>SNAEK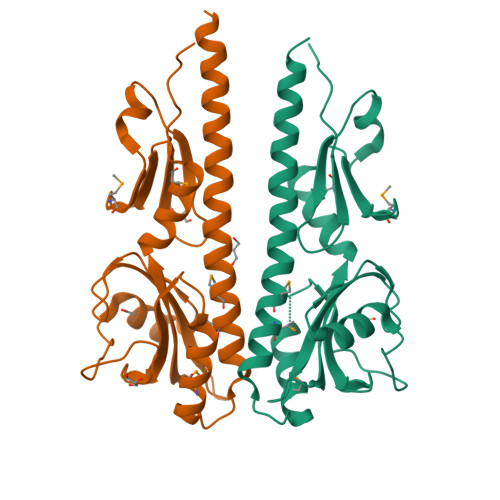EKDTIAAEHKQEASVLLNLHRNKINYLIGETMARMTSLSIAIDRPVDIKKMQSILEKTFDSEPRFSGLYFLNAKGDVTASTTELKTKVNLADASFFIKAKETKKTVISDSYSSRITGQPIFTICVPVLDSKRNVTDYLVAAIQIDYLKNLINLLSPDVYIEVVNQDGKMIFASGQASHAEDQKPVSGYLDDISWNMKVYPNPVTIEELSKSL[2x]>[2x]KHSLPDLPYDYGALEPHINAQIMQLHHSKHHAAYVNNLNVTEEKYQEALAKGDVTAQIALQPAL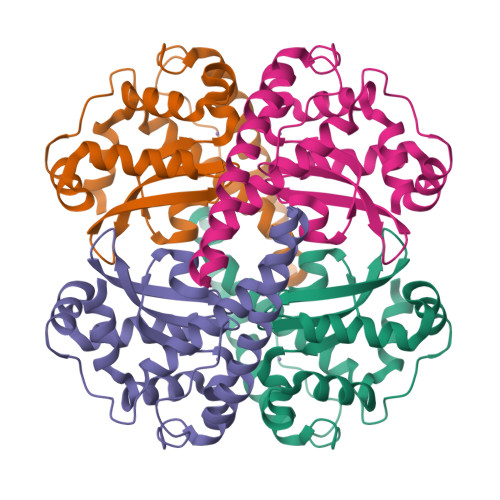KANGGGHINHSIFWTNLSPNGGGEPKGELLEAIKRDFGSFDKFKEKLTAASVGVQGSGWGWLGFNKERGHLQIAACPNQDPLQGTTGLIPLLGIDVWEHAYYLQYKNVRPDYLKAIWNVINWENVTERYMAC>[2x]MADSDPGERSYDNMLKMLSDLNKDLEKLLEEMEKISVQATWMAYDMVVMRT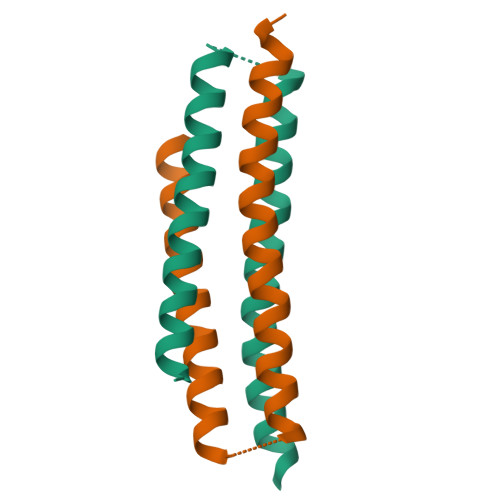NPTLAESMRRLEDAFLNCKEEMEKNWQELLTETKRKQ> MKKNGKSQNQPLDFTQYAKNMRKDLSNQDICLEDGALNHSYFLTKKGQYWTPLNQKALQRGIELFGVGNWKEIN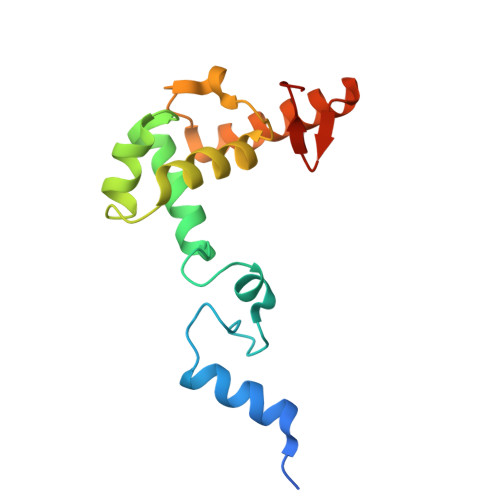YDEFSGKANIVELELRTCMILGINDITEYYGKKISEEEQEEIKKSNIAKGKKENKLKDNIYQKLQQMQ>[12x]MDKTVLDANLDPLKGKTIGVIGYGNQGRVQATIMRENGLNVIVGNVKDKYYELAKKEGFEVYEIDEAVRRSDVALLLIPDEVMKEVYEKKIAPVLQGKKEFVLDFASGYNVAFGLIRPPKSVDTIMVAPRMVGEGIMDLHKQGKGYPVLLGVKQDASGKAWDYAKAIAKGIGAIPGGIAVISSFEEEALLDLMSEHTWVPI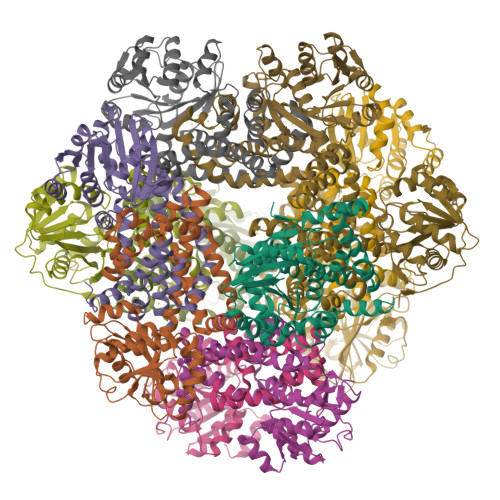LFGAIKACYDIAVKEYGVSPEAALLEFYASGELAEIARLIAEEGIFNQMVHHSTTSQYGTLTRMFKYYDVVRRIVENEAKYIWDGSFAKEWSLEQQAGYPVFYRLWELATQSEMAKAEKELYKLLGRKVKND>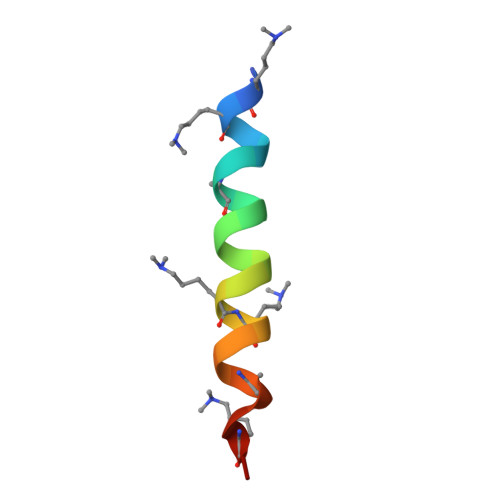 RKKELAKEVIETAKKLIEKLAKEE> GPGKVVKFSYMWTINNFSFCREEMGEVIKSSTFSSGANDKLKWCLRVNPKGLDEESKDYLSLYLLLVSCPKSEVRAKFKFSILNAKGEETKAMESQRAYRFVQGKDWGFKKFIRRDFLLDEANGLLPDDKLTLFCEVSVVQD;> LSASPQPSSV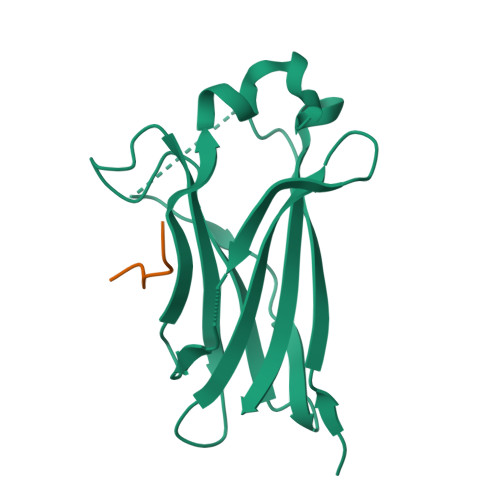APRRPQEPR>[2x]GSQNNECKMVDLR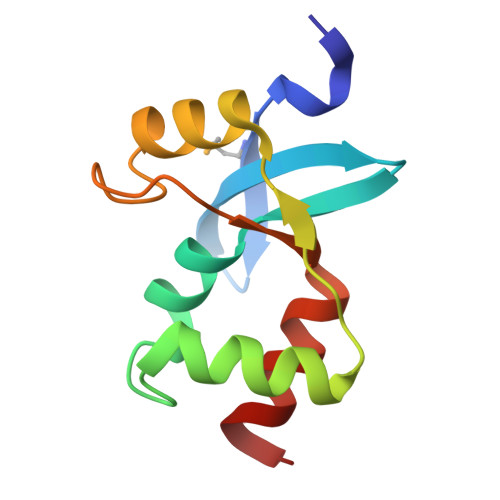GAKVASFTVEGCELICLPQAFDLFLKHLVGGLHTVYTKLKRLEITPVVCNVEQVRILRGLGAIQPGVNRCKLISRKDFETLYNDCTNA[(2R)-2-hydroxy-3-{[(4-oxo-4,5-dihydro-3H-pyrrolo[3,2-d]pyrimidin-7-yl)methyl]amino}propyl]phosphonic 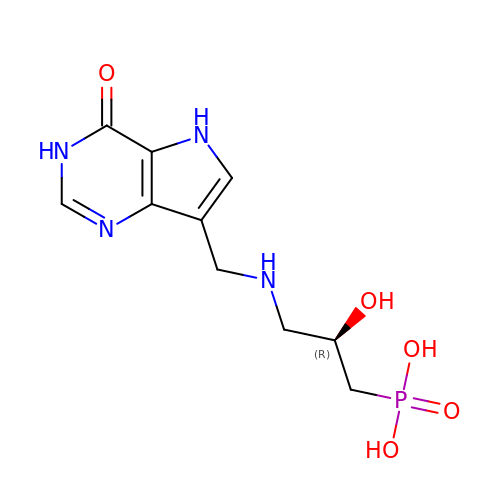acid | C10 H15 N4 O5 P | GLYTVTTVHOOYFN-SSDOTTSWSA-N>[2x]RVAEQARRRAIARAIRQVPIRDILTSPVVTV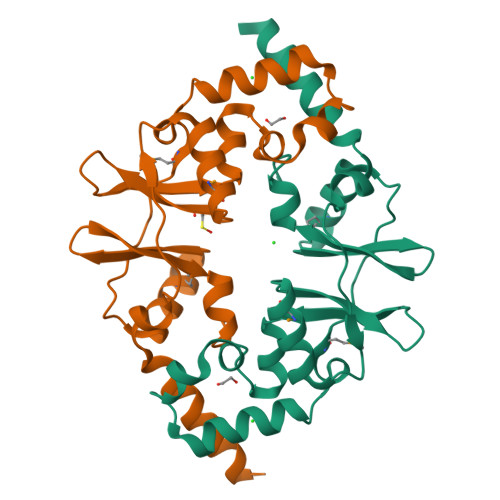REDDTLDAVAKTMLEHQIGCAPVVDQNGHLVGIITESDFLRGSIPFWIYEASEILSRAIPAPEVEHLFETGRKLTASAVMTQPVVTAAPEDSVGSIADQMRRHGIHRIPVVQDGVPVGIVTRRDLLKLLLLEESPVDPD> MVPISPIETVPVKLKPGMDGPKVKQWPLTEEKIKALVEICTEMEKEGKISKIGPENPYNTPVFAIKKKDSTKWRKLVDFRELNKRTQDFWEVQLGIPHPAGLKKKKSVTVLDVGDAYFSVPLDEDFRKYTAFTIPSINNETPGIRYQYNVLPQGWKGSPAIFQSSMTKILEPFAAQNPDIVIYQYMDDLYVGSDLEIGQHRTKIEELRQHLLRWGLTTPDKKHQKEPPFLWMGYELHPDKWTVQPIVLPEKDSWTVNDIQKLVGKLNWASQIYPGIKVRQLSKLLRGTKALTEVIPL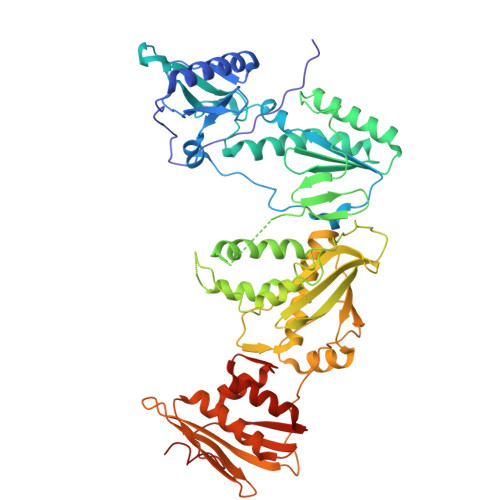TEEAELELAENREILKEPVHGVYYDPSKDLIAEIQKQGQGQWTYQIYQEPFKNLKTGKYARMRGAHTNDVKQLTEAVQKITTESIVIWGKTPKFKLPIQKETWETWWTEYWQATWIPEWEFVNTPPLVKLWYQLEKEPIVGAETFYVDGAANRETKLGKAGYVTNKGRQKVVPLTNTTNQKTELQAIYLALQDSGLEVNIVTDSQYALGIIQAQPDKSESELVNQIIEQLIKKEKVYLAWVPAHKGIGGNEQVDKLV> MPISPIETVPVKLKPGMDGPKVKQWPLTEEKIKALVEICTEMEKEGKISKIGPENPYNTPVFAIKKKDSTKWRKLVDFRELNKRTQDFWEVQLGIPHPAGLKKKKSVTVLDVGDAY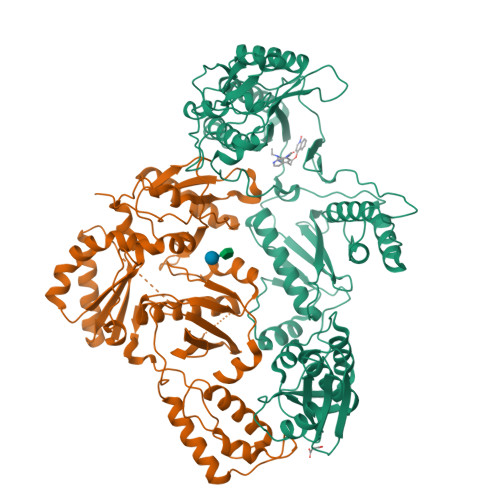FSVPLDEDFRKYTAFTIPSINNETPGIRYQYNVLPQGWKGSPAIFQSSMTKILEPFRKQNPDIVIYQYMDDLYVGSDLEIGQHRTKIEELRQHLLRWGLTTPDKKHQKEPPFLWMGYELHPDKWTVQPIVLPEKDSWTVNDIQKLVGKLNWASQIYPGIKVRQLCKLLRGTKALTEVIPLTEEAELELAENREILKEPVHGVYYDPSKDLIAEIQKQGQGQWTYQIYQEPFKNLKTGKYARMRGAHTNDVKQLTEAVQKITTESIVIWGKTPKFKLPIQKETWETWWTEYWQATWIPEWEFVNTPPLVKLWYQLEKEPIVGAETFYVDGAANRETKLGKAGYVTNRGRQKVVTLTDTTNQKTELQAIYLALQDSGLEVNIVTDSQYALGIIQAQPDQSESELVNQIIEQLIKKEKVYLAWVPAHKGIGGNEQVDKLVSAGIRKVLVPR;> GSPISPIETVPVKLKPGMDGPKVKQWPLTEEKIKALVEICTEMEKEGKISKIGPENPYNTPVFAIKKKDSTKWRKLVDFRELNKRTQDFWEVQLGIPHPAGLKKKKSVTVLDVGDAYFSVPLDEDFRKYTAFTIPSINNETPGIRYQYNVLPQGWKGSPAIFQSSMTKILEPFRKQNPDIVIYQYMDDLYVGSDLEIGQHRTKIEELRQHLLRWGLTTPDKKHQKEPPFLWMGYELHPDKWTVQPIVLPEKDSWTVNDIQKLVGKLNWASQIYPGIKVRQLCKLLRGTKALTEVIPLTEEAELELAENREILKEPVHGVYYDPSKDLIAEIQKQGQGQWTYQIYQEPFKNLKTGKYARMRGAHTNDVKQLTEAVQKITTESIVIWGKTPKFKLPIQKETWETWWTEYWQATWIPEWEFVNTPPLVKLWYQLEKEPIVGAETF>[2x]MVGQIAKEMGLRAYIVGGVVRDILLGKEVWDVDFVVEGNAIELAKELARRH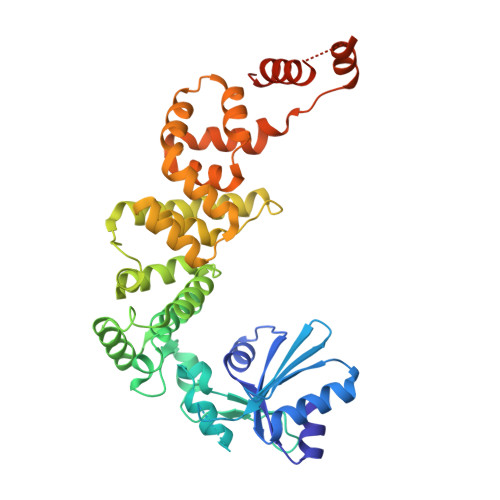GVNVHPFPEFGTAHLKIGKLKLEFATARRETYPRPGAYPKVEPASLKEDLIRRDFTINAMAISVNLEDYGTLIDYFGGLRDLKDKVIRVLHPVSFIEDPVRILRALRFAGRLNFKLSRSTEKLLKQAVNLGLLKEAPRGRLINEIKLALREDRFLEILELYRKYRVLEEIIEGFQWNEKVLQKLYALRKVVDWHALEFSEERIDYGWLYLLILISNLDYERGKHFLEEMSAPSWVRETYKFMKFKLGSLKEELKKAKENYEVYRLLKPLHTSVLLLLMLEEELKEKIKLYLEKLRKVKLPKEKIEELKKQGLKGKELGERIEELKREIMNKIKLAAALEHHHHHH N-[(1S)-1-(2,4-difluorophenyl)ethyl]-3-(5-methyl-1H-pyrazol-3-yl)imidazo[1,2-b]pyridazin-6-amine 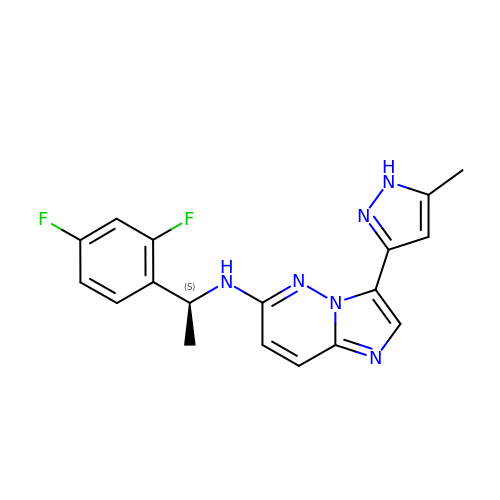| C18 H16 F2 N6 | SMKJDFHRUWJNRS-NSHDSACASA-N>[3x]MKKLTIGLIGNPNSGKTTLFNQLTGSRQRVGNWAGVTVERKEGQFSTTDHQVTLVDLPGTYSLTTISSQTSLDEQIACHYILSGDADLLINVVDASNLERNLYLTLQLLELGIPCIVALNMLDIAEKQNIRIEIDALSARLGCPVIPLVATRGRGIEALKLAIDRYKANENVELVHYAQPLLNEADSLAKVMPSDIPLKQRRWLGLQMLEGDIYSRAYAGEASQHLDAALARLRNEMDDPALHIADARYQCIAAICDVVSN

Structural studies have also illustrated a large conformational change in the G5 loop of the intracellular Ras-type GTPase domain (NFeoB) of the prokaryotic iron transporter FeoB, when comparing crystal structures of apo and nucleotide bound states. The G5 motif is generally comprised of six amino acids with a relatively poor sequence conservation, although the motif invariably forms a loop with electrostatic or hydrophobic interactions with the guanine nucleotide base. We have used the EcNFeoB (Escherichia coli FeoB) protein as a model system because of its clearly resolved conformational change in the G5 loop as revealed by crystal structure analyses. We systematically mutated the residues in the loop to alanine and characterized their biochemical properties in order to determine their individual roles in nucleotide affinity, GTP hydrolysis and GDP release.

Given their drastic biochemical deviations, we also validated the integrity of the S150A and T151A mutants by determining their crystal structures, which illustrated that the mutations did not have any adverse effects on the overall fold of the protein or on the G5 loop. Under experimental conditions, the S150A mutant demonstrated the fastest GTP hydrolysis rate (kcat=0.67 min−1), a rate approximately 1.5 times faster than that of wild-type EcNFeoB. The kon values for the mutant proteins were variable but within the same order of magnitude, with the S150A mutant having the fastest association rate (26±1 μM−1 min−1) and the R154A mutant the slowest (4.3±0.1 μM−1 min−1). The R152A, G153A and R154A mutations did not alter the release rate significantly, while the S150A mutant has a release rate that is approximately 7-fold slower (koff=22.4±0.1 s−1) than that of the wild-type protein. Furthermore, the ITC experimental results showed that the S150A mutant protein had the greatest GDP affinity (Kd=2.0 μM), approximately five times that of wild-type EcNFeoB, which is also in agreement with a decelerated GDP release rate. The StNFeoB protein has, as most other GTPases, an alanine residue at this position. Comparing the structures of GDP bound wild-type StNFeoB and an A143S mutant protein (equivalent to EcNFeoB S150), illustrated that the mutation destabilizes the nucleotide base by altering the hydrogen-bonding network. It is thus likely that this is also the case for the wild-type EcNFeoB protein, while the S150A mutation generates a more stable nucleotide-binding environment. Our results show that the two most important residues for intrinsic affinity and release of GDP are the second (S150) and third (T151) residues of the G5 loop, which are also the two residues exhibiting the largest conformational shift in EcNFeoB (9 and 7 Å, respectively).propionylthiocholine 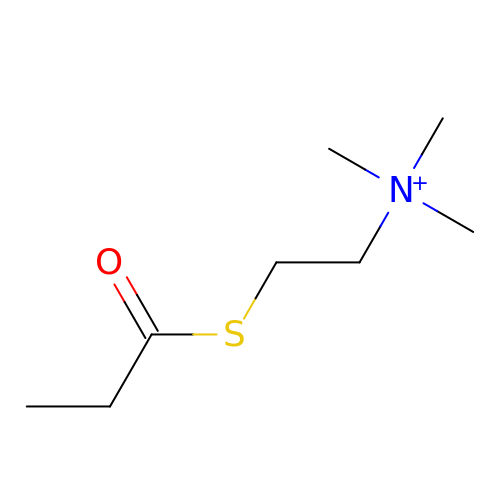| C8 H18 N O S | ILWCNQXVCCMVCY-UHFFFAOYSA-N> AVGPVADNTITDAATSPDGFSRQAVVVNGVTPGPLVAGNIGDRFQLNVIDNLTNHTMLKTTSVHWHGFFQQGTNWADGPAFINQCPISPGHSFLYDFQVPNQAGTFWYHSHLSTQYCDGLRGPFVVYDPNDPHASRYDVDNDDTVITLADWYHTAAKLGPRFPAGADATLINGKGRAPSDTSAELSVIKVTKGKRYRFRLVSLSCDPNFTFSIDGHNLTIIEVDSSNSQPLSVDSIQIFAAQRYSFVLNANQAVDNYWIRANPNFGNVGFN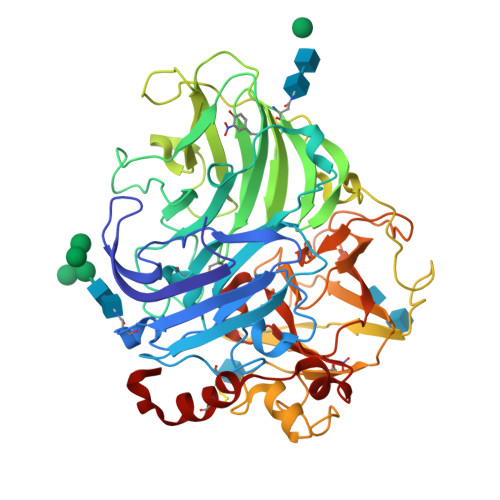GGINSAILRYDGAPAVEPTTNQTTSVKPLNEVNLHPLVSTPVPGSPSSGGVDKAINMAFNFNGSNFFINGASFVPPSVPVLLQILSGAQTAQDLLPSGSVYVLPSNASIEISFPATAAAPGAPHPFHLHGHTFAVVRSAGSTVYNYSNPIFRDVVSTGTPAAGDNVTIRFLTNNPGPWFLHCHIDFHLEGGFAVVQAEDVPDVKATNPVPQAWSDLCPTYDANAPSDQ> MSPILAKNIVYVAQIKGQITSYTYDQFDRYITIAEQDNAEAIIIELDTPGGRADAMMNIVQRIQQSKIPVIIYVYPPGASAASAGTYI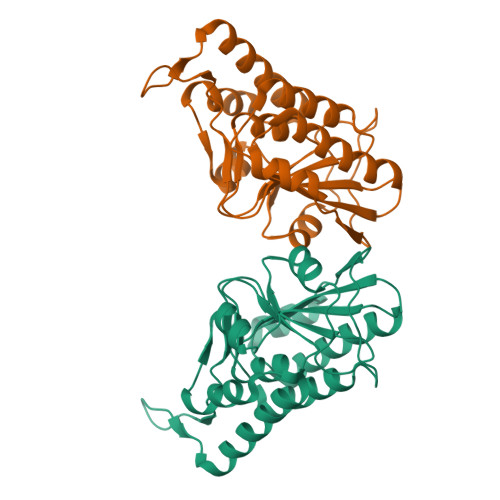ALGSHLIAMAPGTSIGACRPILGYSQNGSIIEAPPAITNYFIAYIKSLAQESGRNATIAEEFITKDLSLTPEEALKYGVIEVVARDINELLKKSNGMKTKIPVNGRYVTLNFTNVEVRYLAPSFKDKLISYITDLEHHHHHH>[2x]MIKAVVFDAYGTLFDVQSVADATERAYPGRGEYITQVWRQKQLEYSWLRALMGRYADFWS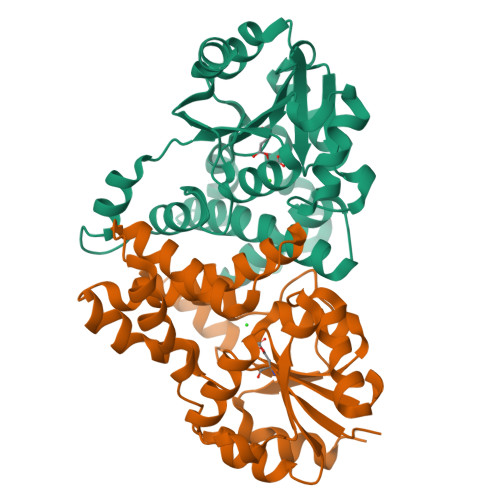VTREALAYTLGTLGLEPDESFLADMAQAYNRLTPYPDAAQCLAELAPLKRAILSNGAPDMLQALVANAGLTDSFDAVISVDAKRVFKPHPDSYALVEEVLGVTPAEVLFVSSNGFDVGGAKNFGFSVARVARLSQEALARELVSGTIAPLTMFKALRMREETYAEAPDFVVPALGDLPRLVRGMAGAHLAPAV> MTGIPTVTARPWTQRPRAENSTTNPTYFFTFGDSYSQTGFSASGTQPSASNPMGNPDLGIGTTTNGPNWIGYLTTTENASLVLSYNLAAGGATIDNALVPAYPGDLASQFRLFEDVYADKPASAPWSAEDAVFGVWIGDNDIGNAYYSTDAETYTP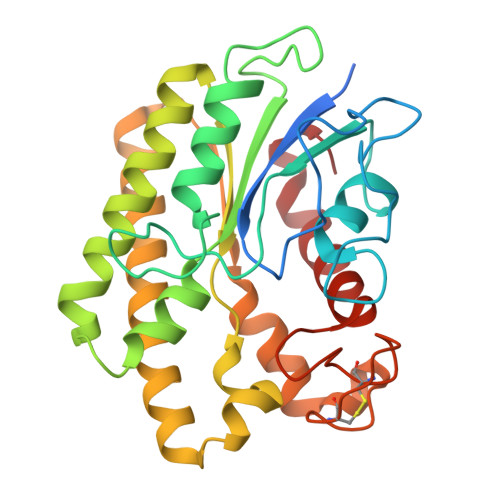KLISRLESLVEEVYKNGGRKFLFLNVPPTSRSPLFLEQGEEVVKQHAEYLSVYNENLEGMVDDFTKKKGDVTTVLYDSWSFMTKILDDPTAYGFPDATCINDDGTSCIWWDNYHPGMKYHLLQAEDMKPKLRKLGGW>MRDLYRNTNTFMIRTPIFSIDNYYEFFRKDGESDKIKDRLLEICNNSVFREAILVSSKSLYSTIIDFCDGKEIKKFDYFLQSIYKYLIRMSMRPTPFGLFSGVDFGKYAEETVISYENDNFKKFARPDLEWIIKIVKELEDNHYKNLTFKINDSIFIKGERALLIHSTDKEDNNRIGEISIRATKPFMRTYDLAKDGIEYNKLKYI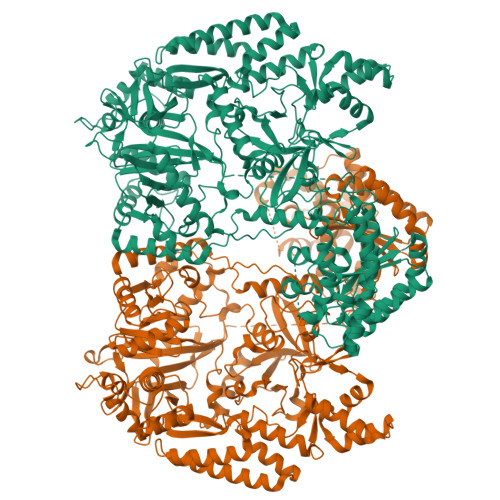LIDEYSIEDESKIDNFLKQLIEREFLISNLRPPLTVLDQFDYLINEVKKAEIEIPLVDELTEIKEKLKLYNETPVGAGEETYLELYKKMESVANVKNILQVDMKLNLRDKKINKKIISDVNDLMNILLDLSMSIENPEPFLSKYKQEFIEKYGQDREISLLEMLDNDIGIGPPMNYERPRNNRSLDVSVNELLDNNVRDYFMEKYFQALKTNSRNIAIRDDEIKNLELQKIDYENIPDSLEINLLVKNKSEDNLSDEFQYYIGPNLGSTSAGKSFGRFSHMMSEPKKFFEELDERNIELIDSEEYVTCEISYLPSEVRNANVTRNIHSSEYEMSLFTNGSKDNLYRIKLNDIYIGLENNTFYAKSKTLNKKLLLTINNMLNPQTAPNAIRFLNDISLDEKKLWYKFVWSDVYKDFSYIPAIKYKNFVIMPETWKMNKINMKINKKTEFNEFKNQFNDYRIKYGVPQYVYITFADNRILLNLDDEQCVKILYHECKNSFNEIILNSYEEEGVNIVKESHKDYICELVIPLTKIKQETISDKVSARMLSSDISSLSKERVKDPFDEWLYIKLYGISSNVDDLIAYYISEFCNELVEEEIISKYFFMRYVDPEQHIRLRLNSSQEKLLMIYPKIREWLSMIRKKGLMTYFSIDSYDREIERYGGIELINIAEKVFFFDSIVTEDILRAKREGSFDFCDEIIGMISVVHYMESFGLPYAKQVEFLRSQVSSSEYREDFKQKRTEYMKLCNSNKDWEGLRESEEGNILIEILNKRRKIIEYYGNKVRENEEVSTDLSILDSIIHLNCNRMFGIDREFEKKVRALASHALYALKHFKS[2x]> MRKFIIVKNVKVDGIN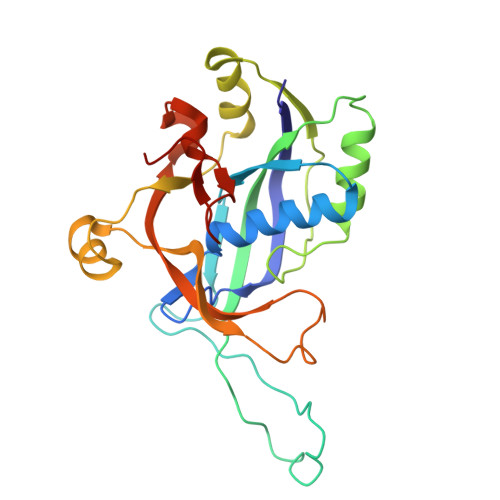AKSSDITVGMPPATTFCGLGETMSIKTGIVVKAVSYGSVKFEVRGSRFNTSVTKFAWQDRGNGGKANNNSPIQPKPLADGVFTLCFEVEWEDCAEVLVDKVTNFINTARIAGGTIASFNKPFVKVAKDAEELASVKNAMMPCYVVVDCGVEVNIFEDAVNRKLQPMVNGYKKLEKIVDNKHMRDKFTPAYLATPTYTMIGYKMVSNVDNFDQALWQYGENTKVKTIGGIYND>MQIKAGLIWMNGAFVPQEEAKTSVLSHALHYGTSVFEGIRAYETAKGPAIFRLKEHVKRFYNSAKVLRMEIPFAPEELEEAIKEVVRRNGYRSCYIRPLAWMGAKALGVNPLPNNPAEVMVAAWE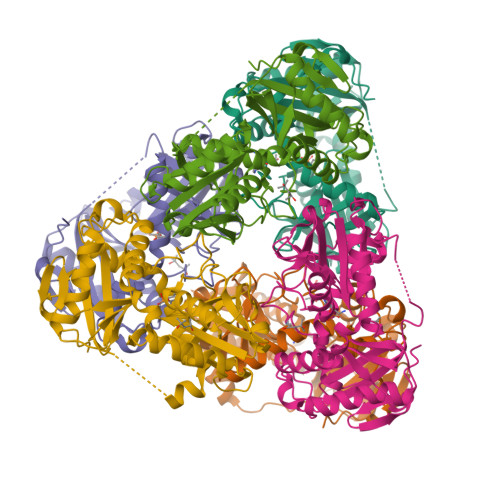WGAYLGEEAVRKGARLITSSWARFPANVMPGKAKVGGNYVNSALAKMEAVAAGADEALLLDEEGYVAEGSGENLFFVRDGVIYALEHSVNLEGITRDSVIRIAKDLGYEVQVVRATRDQLYMADEVFMTGTAAEVTPVSMIDWRPIGKGTAGPVALRLREVYLEAVTGRRPEYEGWLTYVNGQ[6x]>MNKNNTKLSTRALPSFIDYFNGIYGFATGIKDIMNMIFKTDTGGDLTLDEILKNQQLLNDISGKLDGVNGSLNDLIAQGNLNTELSKEILKIANEQNQVLNDVNNKLDAINTMLRVYLPKLTSMLSDVMKQNYALSLQIEYLSKQLQEISDKLDIINVNVLINSTLTEITPAYQRIKYVNEKFEELTFATETSSKVKKDGSPADILDELTELTELAKSVTKNDVDGFEFYLNTFHDVMVGNNLFGRSALKTASELITKENVKTSGSEVGNVYNFLIVLTALQAKAFLTLTTCRKLLGLADIDYTSIMNEHLNKEKEEFRVNILPTLSNTFSNPNYAKVKGSDEDAKMIVEAKPGHALIGFEISNDSITVLKVYEAKLKQNYQVDKDSLSEVIYGDMDKLLCPDQSEQIYYTNNIVFPNEYVITKIDFTKKMKTLRYEVTANFYDSSTGEIDLNKKKVESSEAEYRTLSANDDGVYMPLGVISETFLTPINGFGLQADENSRLITLTCKSYLRELLLATDLSNKETKLIVPPSGFISNIVENGSIEEDNLEPWKANNKNAYVDHTGGVNGTKALYVHKDGGISQFIGDKLKPKTEYVIQYTVKGKPSIHLKDENTGYIHYEDTNNNLEDYQTINKRFTTGTDLKGVYLILKSQNGDEAWGDNFIILEISPSEKLLSPELINTNNWTSTGSTNISGNTLTLYQGGRGILKQNLQLDSFSTYRVYFSVSGDANVRIRNSREVLFEKRYMSGAKDVSEMFTTKFEKDNFYIELSQGNNLYGGPIVHFYDVSIK[4x]

In addition, Bt secretes to the medium numerous vegetative insecticidal proteins (Vip) that have been classified into three different families. Notably, members of the Vip3 family have shown to have a broad-spectrum activity against Lepidoptera4 and, since they target binding sites different to those of Cry proteins in the insect membranes, they are considered a good complement to the action of these toxins. Vip3 proteins are synthesized in an inactive state, as protoxins, and they require to be activated by proteases present in the midgut tract of the insect. To shed light on some of these questions, we have determined the near-atomic resolution structures of Vip3Aa in the protoxin and activated states by cryo-electron microscopy (cryo-EM).

We therefore decided to solve the three-dimensional structure of Vip3Aa after trypsin treatment. Activated Vip3Aa shows the same domain organization described in the protoxin state, and domains II–V maintain a similar global architecture. Domain I, however, suffers a large conformational change that remodels the apex of the pyramid into a ~200 Å-long needle. In particular, three antiparallel N-terminal helices (α2–α4) undergo a set of rotations, in a manner akin to a folding cane, to form a long continuous helix that assembles into a parallel four-helical coiled-coil in the digested Vip3Aa tetramer. The cryo-EM analysis shows that the coiled-coil is relatively ordered starting at the beginning of α2 (~D45), and that the flexible end is formed by the most N-terminal region of the protein, which contain the residues forming the first alpha helix in the protoxin state. Close examination of the structure of the toxin revealed that the coiled-coil of Vip3A, which resembles other four-helix bundles such as the SNARE complex (RMSD of 3.4 Å for 232 residues), extends ~160 Å and that the average internal radius of the modeled section was 1.46 Å. Interestingly, comparative analysis of different structures, like that of the Sendai virus P protein, have shown that hydrophilic residues found in these positions—known as N@d layers—can bind ions and water molecules in the central cavity of the tetrameric coiled-coil. Although the resolution of the cryo-EM reconstruction does not allow visualization of water molecules, there is a clear peak of density coordinated by four symmetry related asparagines (N163) that, based on the buffer composition (5 mM MgCl2), was assigned to a magnesium ion. Domain I is indeed retained after protease digestion and stays tightly bound to the core of the protein through interactions with domain II, forming an essential part of the active toxin. Notably, the coiled-coil observed upon trypsin digestion forms a 160 Å-long dipole that can accommodate small ions in the inner cavity and, therefore, the dimension of this four-helix needle would be sufficient to reach and pierce the lipid bilayer.>PLGSVRWARALYDFEALEEDELGFRSGEVVEVLDSSNPSWWTGRLHNKLGLFPANYVAPMMR[2x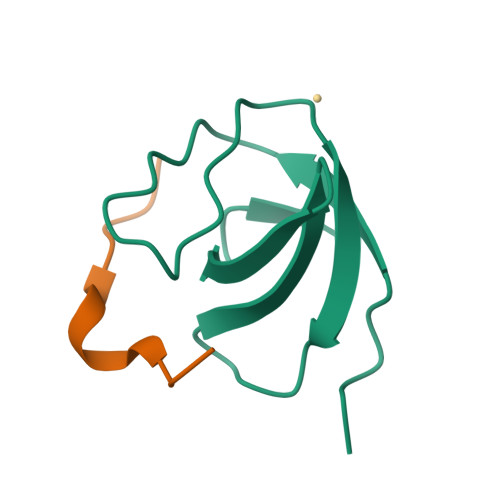];>[2x]PAPSIDRSTKPPL Here, we investigated a new Class II metal aldolase from the p-hydroxyphenylacetate degradation pathway in Acinetobacter baumannii, 4-hydroxy-2-keto-heptane-1,7-dioate aldolase (AbHpaI), which has various properties suitable for biocatalysis, including stereoselectivity/stereospecificity, broad aldehyde utilization, thermostability, and solvent tolerance. For Class II metal aldolases, the enzyme uses a divalent metal ion (M2+) as a cofactor for substrate binding and stabilization of an enolate intermediate, which allows the reaction to proceed through C-C bond formation or cleavage. Each protomer contains eight β/α motifs of a TIM barrel fold with an additional α-helix (residues 6–11; N-helix) at the N-terminus. Three protomers are associated in a tight trimeric structure to generate three catalytic pockets, and the trimer is dimerized to form a stable and rigid hexamer with 35% buried area.

Notably, the use of Zn2+ by AbHpaI as a native cofactor is distinct from other enzymes in this class. Zn2+ binds to AbHpaI in an octahedral coordination with six chelating atoms consisting of the pyruvate core, Glu151, Asp177, and two water molecules (WA and WS1), so does the geometry of Co2+, Mn2+, and Mg2+, which differs from Zn2+ tetrahedral coordination commonly found in aldolase and nonaldolase enzymes. Notably, Glu151 and Asp177 in the Zn2+, Co2+, or Mn2+ complexes were more rigid than those of apo-AbHpaI, as reflected by temperature factors (B-factors) of the crystal structure. AbHpaI has three and sevenfold greater affinity for Zn2+ binding over Co2+ and Mn2+, respectively, while the Kd of Mg2+ and Ca2+ to AbHpaI could not be determined. The Tm values of AbHpaI were enhanced by 5.7, 3.4, and 1.7 °C upon binding to Zn2+, Co2+, and Mn2+, respectively. Consequently, the result suggested that Zn2+ enhances the thermostability of AbHpaI, the highest among all types of AbHpaI•M2+ enzymes. Zn2+ binding can enhance stereoselectivity in aldol reactions and enzyme thermostability.

>MVNTVNYFKQKLKTEQQIGMWVGLADGYCAEIAANVGYDWLLIDGEHAPNDVRSILAQLQSIAAYPSQAVVRPVSGDVPLIKQLLDIGAQTLLIPMVESAEQAELMVKATRYPPEGIRGVGAALARASRWNNISDYLQTADEQICLLVQVESKKGLDNLDEILNVDGVDGIFIGPADLSAALGYRGNPGHEFVQNIIVQTIQKIRAAGKAAGILSADEKLAKQYLELGTEFVAVGVDTSLLMKSMKQLLSKFKNVDGPVSTSPSVY[3x]Belinostat | C15 H14 N2 O4 S | 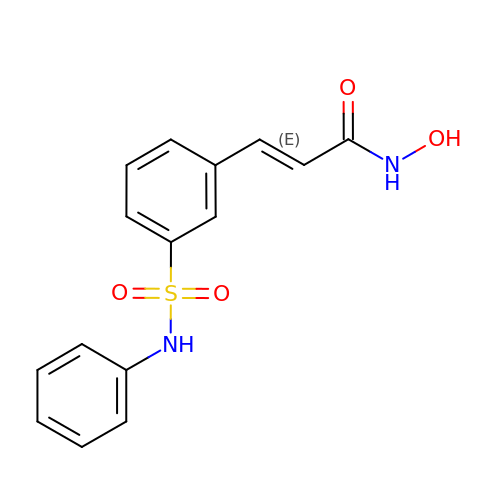NCNRHFGMJRPRSK-MDZDMXLPSA-N>[2x]MQIPASEQETL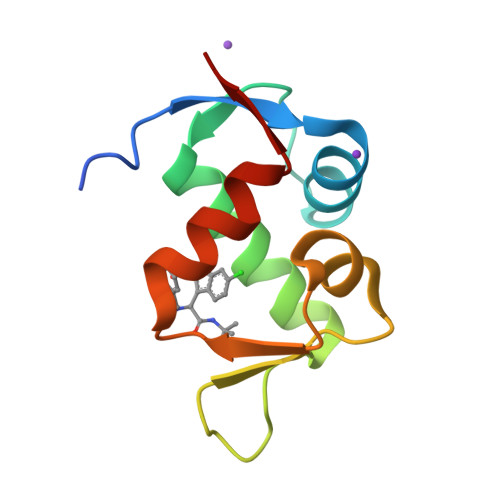VRPKPLLLKLLKSVGAQKDTYTMKEVLFYLGQYIMTKRLYDEKQQHIVYCSNDLLGDLFGVPSFSVKEHRKIYTMIYRNLVVVN>SGPNGGVCPVLIYLCRRDSDCPGECICLGNGYCG[4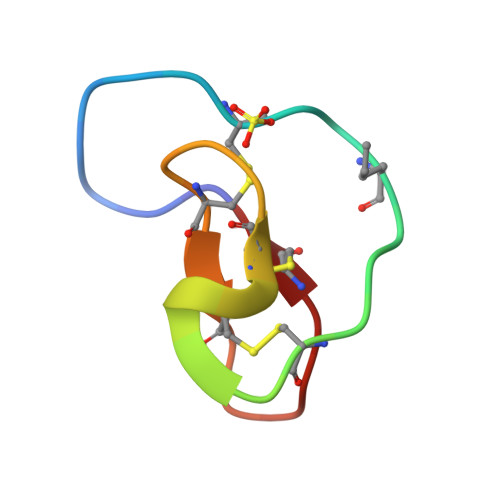x]>[2x]GPLGSGRPTPRSRASAKARAKLLAEVEARDPW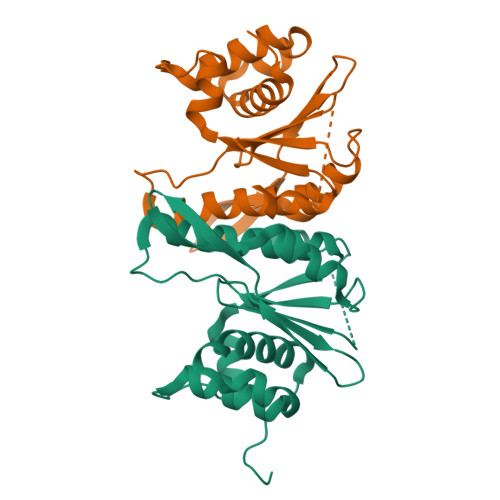LASLSLLPTDDIPSADATTNGWVIGVDPDIGGAIAVLSPDGSSQVFDNPFVHIVVSEVIRKRLDTKSIIQLLRGLDAPPGTTAYIEKSSPFPTDGKQGWWSTGFSYGLWIASLVASGFSVVPIASQTWKAYFGLMRSETPKDDSRQAASILFPDKDQSLKLKKHHGRAEALLLAAYGKGLVLPSGKFSKTSV5-bromanyl-N-methyl-1H-indazole-3-carboxamide 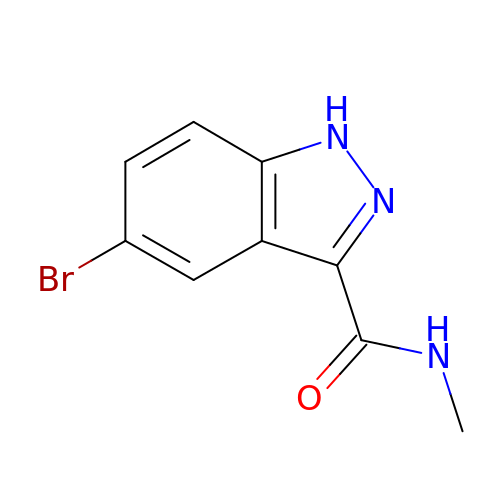| C9 H8 Br N3 O | LZKFBFNVDKRHMH-UHFFFAOYSA-N> TGRPEWIWLALGTALMGLGTLYFLVKGMGVSDPDAKKFYAITTLVPAIAFTMYLSMLLGYGLTMVPFGGEQNPIYWARYADWLFTTPLLLLDLALLVDADQGTILALVGADGIMIGTGLVGALTKVYSYRFVWWAISTAAMLYILYVLFFGFTSKAESMRPEVASTFKVLRNVTVVLWSAYPVVWLIGSEGAGIVPLNIETLLFMVLDVSAKVGFGLILLRSRAIFGEA

Bacteriorhodopsin (bR) is a light-driven proton pump found in the plasma membrane of a halophilic archaeon, Halobacterium salinarum. bR is one of the most extensively studied membrane proteins, and has been investigated using a wide range of experimental and theoretical approaches. Seven transmembrane helices (A–G) surround a retinal molecule which is covalently bound to the side chain of Lys216 in helix-G with the Schiff base (SB) linkage. The proton path is composed of charged residues such as Arg82, Asp85, Asp96, Glu194, Glu204, Asp212 and SB. In order to elucidate previously veiled features of the retinal chromophore as well as proton-path forming residues, we performed high-resolution X-ray crystallographic analysis of bR in the ground state.

A dataset with a resolution of 1.29 Å was obtained from a single crystal. The dose to each irradiated position in the dataset was estimated to be 0.1 MGy. The structures were almost identical to each other, with a root mean square deviation (rmsd) of ~0.1 Å in the superimposition of all Cα atoms. Therefore, we mainly present the structure from Dataset I in this paper, while geometric parameters are derived as the averaged values of the three structures. The structure consists of 229 residues, one retinal, four lipids and 30 waters. The structure contains the loop EF (Thr157 − Glu161), which is absent in 1C3W10. In addition, multiple conformations were observed for 8 residues. The high-resolution electron density map enables us to recognize the respective atomic positions of the retinal molecule which is in the all-trans conformation by means of light adaptation before freezing. Our study reveals that the side chain of Glu204 in the proton release group at the extracellular side of bR takes two conformations. The occupancies of the two conformations are refined to be 0.55 and 0.45.>[2x]MFLRIDRLQIELPMPKEQDPNAAAAVQALLGGRFGEMSTLMNYMYQSFNFRGKKALKPYYDLIANIATEELGHIELVAATINSLLAKNPGKDLEEGVDPASTPLGFAKDVRNAAHFIAGGANSLVMGAMGEHWNGEYVFTSGNLILDLLHNFFLEVAARTHKLRVYEMTDNPVAREMIGYLLVRGGVHAAAYGKALESLTGVEMTKMLPIPKIDNSKIPEAKKYMDLGFHRNLYRFSPEDYR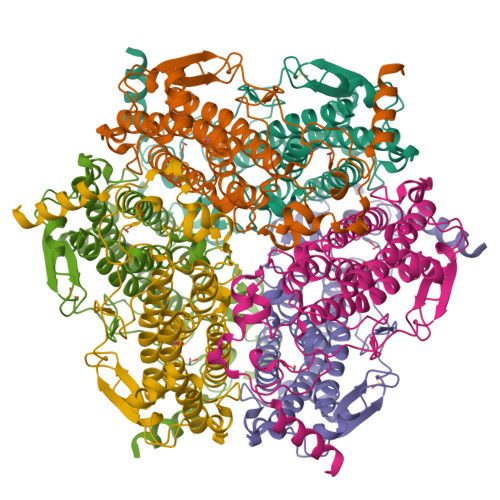DLGLIWKGASPEDGTEVVVVDGPPTGGPVFDAGHDAAEFAPEFHPGELYEIAKKLYEKAK>TDENQTIQNDSSSSLTQVNTTMSVQMDKKALLCCFSSPLINAVLITWIIKHRHLPSCTIAYNLDKKTNETSCLGRNITWASTPDHSPELQISAVALQHEGTYTCEIVTPEGNLEKVYDLQVLVPPEVTYFPGKNRTAVCEAMAGKPAAQISWTPDGDCVTKSESHSNGTVTVRSTCHWEQNNVSVVSCLVSHSTGNQSLSIELSQGTMTTPRSTRHHHHHH[3x]

CD200 is a widely distributed membrane glycoprotein that regulates myeloid cell activity through its interaction with an inhibitory receptor (CD200R). CD200R is a member of a “paired receptor” family as in addition to this inhibitory receptor there is one very closely related gene with activating potential in humans and several in mice (Akkaya and Barclay, 2010; Wright et al., 2003). We report X-ray crystallography structures for the inhibitory CD200R, the activating receptor CD200RLa, and a complex between CD200R and CD200.

The structure of CD200RLa was solved after phase determination using crystals soaked in gadolinium chloride solution because molecular replacement (MR) phasing was unsuccessful. The structure of CD200RLa is very similar to that of CD200R, as expected due to their high amino acid sequence identity in their extracellular regions (86%). Superposition of the V-like domains of CD200R and CD200RLa reflects these differences with an average root mean square deviation (rmsd) of 2.05 Å over 106 Cα atoms whereas the C2-like domains superimpose with an rmsd of 0.6 Å over 80 Cα atoms. Despite CD200RLa sharing a high amino acid sequence identity with CD200R in the V-like domain (84% identity in residues 1–123), it gives minimal binding to CD200 (50-fold lower affinity; Wright et al., 2003). Comparison of the CD200R and CD200RLa sequences does not show simple changes in the contact residues that might explain why the activating receptor CD200RLa does not bind CD200, implying indirect effects. To investigate this, the structure of the V-like domain of CD200RLa was superimposed onto CD200R in complex with CD200. Residues 63 and 66 in the C′C″ loop differ between CD200R and CD200RLa and are at the periphery of the interaction with K63, making contact with F96 and L30 of CD200. Substitution of F114 for Leu in CD200RLa seems to cause the side chain of F36 to flip in the opposite direction into the core of the domain. This in turn leads to the destabilization of the NH2 region of CD200RLa and therefore disruption of the CD200 binding interface. Thus both regions are important in explaining why the CD200RLa does not bind CD200 and this argument was strengthened by the analysis of a CD200RLa triple mutant combining both regions (N63K, K66T, and L114F) that binds CD200 with a similar affinity as CD200R.The DNA damage response in mycobacteria is controlled by the heterodimeric transcription factor PafBC, a member of the WYL domain–containing protein family. PafB and PafC each feature an N-terminal HTH domain, followed by the WYL domain and a WYL C-terminal extension (WCX) domain involved in heterodimer formation. Here, we demonstrate that the binding of single-stranded DNA (ssDNA) to the WYL domains of PafBC activates the transcription factor.

In our structure, the WYL domains are positioned diametrically, forming the broadest part of the heterodimer. They connect to the C-terminal WCX domains via flexible linkers providing additional flexibility to the WCX domains. The ferredoxin-like fold of the two WCX domains from MsmPafBC reported here, as well as their interaction with each other, is structurally similar (root mean square deviation = 2.04 Å) to the WCX domains of AauPafBC solved by x-ray crystallography. In our RNAP-bound structure of PafBC, the previously proposed ligand-binding grooves of the WYL domains are oriented toward the WCX domains. In the surface representation of the refined PafBC model, a distinct tunnel is visible between the WYL and WCX domains, extending across the entire heterodimer. The Fo-Fc difference density map revealed extra density within this tunnel, linking the WYL domains of PafB and PafC. The arginine residues (PafB: R211/R214 and PafC: R201/R204), which are essential for ssDNA binding to PafBC, are oriented toward this additional density, substantiating its identity as the ssDNA ligand. These observations demonstrate that our structure captured PafBC in an active state, complexed with ssDNA. Although the overall fold of PafB and PafC is similar, the distance between the WYL and WCX domains in PafB is considerably larger than the corresponding distance in PafC. Although the lower resolution of the ssDNA density precludes structural modeling, we show that, instead of two ssDNA molecules binding to the two PafBC WYL domains, a single ssDNA molecule extends across the heterodimer and contacts both WYL domains simultaneously.

> GLSAVSKVERLMNLVIALLSTRTYLPAEKIRTTVAGYADSPSDEAFSRMFERDKNELRDLGIPLETGRVSKWDSTEGYRINRDSYALPPIGLTADEAAAVAVATQLWQSPELVTATQNAVLKLRAAGVDVDADGVGVAIASTATLPGVRGSEEVLQSLLSAIDEGRAVQFEHRPSRSADYTTRTVEPWGVVTHRGRWYLVGHDRDREDTRTFRLSRISAAARPIGPAGAVQKPQDVNLRDIVRRAVAEQPTGERARIWIAGGRATALRRQAVTSTPRTIGGRAGEEITVDIGTWDRLAREIASYGSDAVALEPSSLRDDVVERLRAHAAGGER;> MSQVSTRLVRLLNMVPYFQANPKVTRAEAAAALGVTGKQLDADLDQLWMCGLPGYSPGDLIDFDFVGDTIEVTFSAGVDHPLRLTSTEATGILVALRALVDVPGMVDPEAARSAIAKIESAVGSQRAVVEGITEDTSAEPGAAATVRTAVRENRALTLEYYSASRDSLATRTVDPIRVVLVGDNSYLEAWCRSAEAVRLFRFDRIVDAQLLDDPAAPPPPAVAAGPDTSLFDADPSLPSATLLIGAAAAWMFDYYPLRDITERPDGSCEATMTYASEDWMARFILGFGAEVQVLAPESLATRVRQAAEAALQAYARCV>[2x]APQQINDIVHRTITPLIEQQKIPGMAVAVIYQGKPYYFTWGYADIAKKQPVTQQTLFELGSVSKTFTGVLGGDAIARGEIKLSDPTTKYWPELTAKQWNGITLLHLATYTAGGLPLQVPDEVKSSSDLLRFYQNWQPAWAPGTQRLYAHSSIGLFGALAVKPSGLSFEQAMQTRVFQPLKLNHTWINVPPAEEKNYAWGYREGK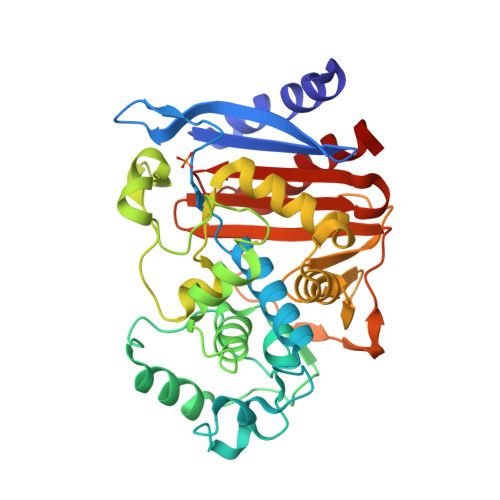AVHVSPGALDAEAYGVKSTIEDMARWVQSNLKPLDINEKTLQQGIQLAQSRYWQTGDMYQGLGWEMLDWPVNPDSIINGSDNKIALAARPVKAITPPTPAVRASWVHKTGATGGFGSYVAFIPEKELGIVMLANKNYPNPARVDAAWQILNALQ> MAFNKDQDYWANIFVTPDFLSVETYSGLGMTGRDPLFSPRLLQPDVDDK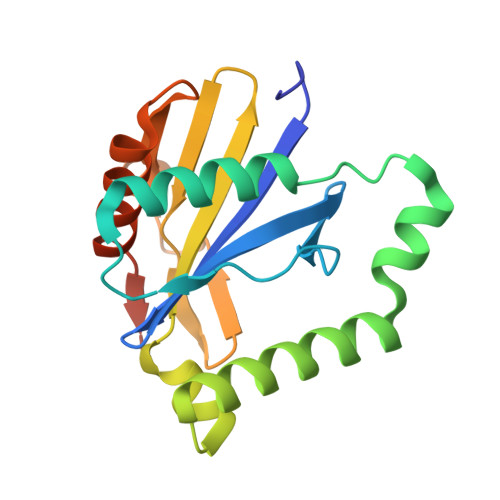SLGEEILQALSDSRTLDVLEERVAFFDLEKSKEQYAAWIATLMEKYGYRTKRALFKNMKKVGIHLVNDVITIRPSFHEKLEAWSGNRINESDYVVLPADSSPTEIGSGLRLALSRCKGTSLEHHHHHH> MDGVHDLAGVQGFGKVPHTVNADIGPTFHAEWEHLPYSLMFAGVAELGAFSVDEVKYVVERMEPRHYMMTPYYERYVIG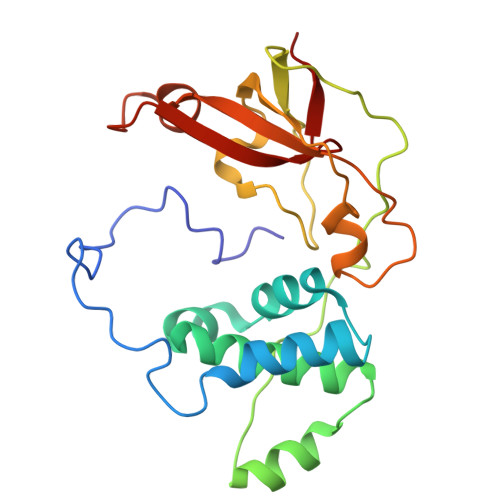VATLMVEKGILTQDELESLAGGPFPLSRPSESEGRPAPVETTTFEVGQRVRVRDEYVPGHIRMPAYCRGRVGTISHRTTEKWPFPDAIGHGRNDAGEEPTYHVKFAAEELFGSDTDGGSVVVDLFEGYLEPAA3-ETHYL-6-{[(4-FLUOROPHENYL)SULFONYL]AMINO}-2-METHYLBENZOIC ACID | C16 H16 F N O4 S | 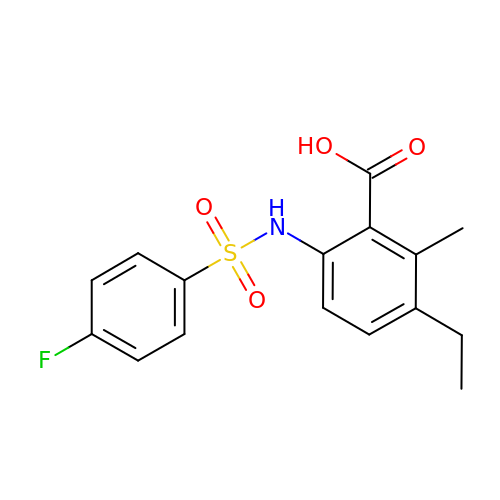MGUQWAOYPINSIT-UHFFFAOYSA-N> MGSSHHHHHHSQDPNSMPDNTIQWDKDADGIVTLTMDDPSGSTNVMNEAYIESMGKAVDRLVAEKDSITGVVVASAKKTFFAGGDVKTMIQARPEDAGDVFNTVETIKRQLRTLETLGKPVVAAINGAALGGGLEIALACHHRIAADVKGSQLGLPEVTLGLLPGGGGVTRTVRMFGIQNAFVSVLAQGTRFKPAKAKEIGLVDELVATVEELVPAAKAWIKEELKANPDGAGVQPWDKKGYKMPGGTPSSPGLAAILPSFPSNLRKQLKGAPMPAPRAILAAAVEGAQVDFDTASRIESR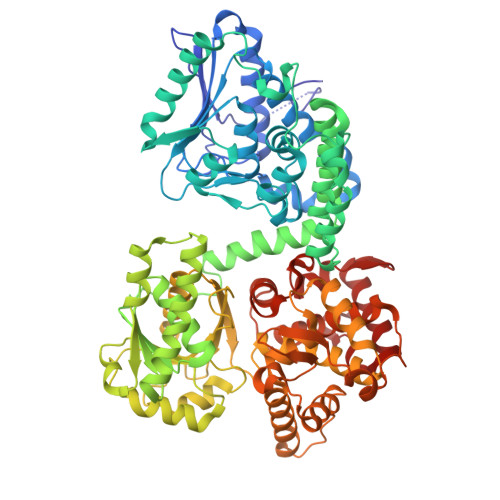YFASLVTGQVAKNMMQAFFFDLQAINAGGSRPEGIGKTPIKRIGVLGAGMMGAGIAYVSAKAGYEVVLKDVSLEAAAKGKGYSEKLEAKALERGRTTQERSDALLARITPTADAADFKGVDFVIEAVFENQELKHKVFGEIEDIVEPNAILGSNTSTLPITGLATGVKRQEDFIGIHFFSPVDKMPLVEIIKGEKTSDEALARVFDYTLAIGKTPIVVNDSRGFFTSRVIGTFVNEALAMLGEGVEPASIEQAGSQAGYPAPPLQLSDELNLELMHKIAVATRKGVEDAGGTYQPHPAEAVVEKMIELGRSGRLKGAGFYEYADGKRSGLWPGLRETFKSGSSQPPLQDMIDRMLFAEALETQKCLDEGVLTSTADANIGSIMGIGFPPWTGGSAQFIVGYSGPAGTGKAAFVARARELAAAYGDRFLPPESLLS>[2x]MGHHHHHHMYTDLKDKVVVITGGSTGLGRAMAVRFGQEEAKVVINYYNNEEEALDAKKEVEEAGGQAIIVQGDVTKEEDVVNLVQTAIKEFGTLDVMINNAGVENPVPSHELSLDNWNKVIDTNLTGAFLGSREAIKYFVENDIKGNVINMSSVHEMIPWPLFVHYAASKGGMKLMTETLALEYAPKGIRVNNIGPGAMNTPINAEKFADPVQRADVESMIPMGYIGKPEEVAAVAAFLASSQASYV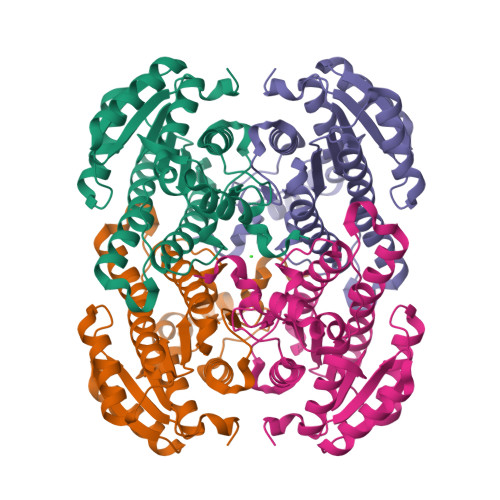TGITLFADGGMTKYPSFQAARG Stx2a holotoxin is a ribosome-inactivating protein (RIP), which belongs to a family of AB5 toxins, consisting of a monomeric A subunit (Stx2A) and a pentameric B subunit (Stx2B). The catalytic A1 subunit of Stx2a (Stx2A1) interacts with the ribosomal P-stalk for loading onto the ribosome and depurination of the sarcin–ricin loop, which halts protein synthesis. The P-stalk is composed of five P-proteins, namely uL10 protein (former name P0) forming the base of the stalk, and two P1–P2 heterodimers, each binding to uL10 (9, 10). Stx2A1 (15, 16) as well as other RIPs bind to the conserved CTDs, with a prominent role of the CTDs from the P1 proteins.

Here, the state-of-the-art instrumentation and multiple software processing platforms were used to determine a 4.1 Å cryo-EM structure of the 72 kDa Stx2a in complex with the ribosomal P-stalk, with local resolutions in the range of 3.5 to 7.5 Å. Stx2A, denoted as chain A, is composed of two fragments, namely a catalytic Stx2A1 fragment consisting of the N-glycosidase active site and the P-stalk CTD-binding site, and Stx2A2 composed of an α-helix, which inserts into the channel formed by a pentameric ring of Stx2B. The structure reveals the presence of a density associated with Stx2a in the region identified earlier as the binding site for the CTD. This density can be fitted with the C-terminal six amino acids from a single P-protein of the P-stalk, denoted as chain P. The cryo-EM structure unveils that the six amino-acid peptide (GFGLFD) from the CTD interacts with Stx2a. The CTD-binding pocket is located on the opposite side of the Stx2a surface than the active site, and it is formed by α-helices: A, F, I, and loop 1 spanning residues Pro27–Ser39. The binding interface involves Stx2a residues previously implicated in the P11 binding by the X-ray structure and mutational analysis, such as Asn18, Thr35, Thr36, Ser229, Leu232, and the conserved Arg172, Arg176, and Arg179. Importantly, the cryo-EM structure reveals novel previously unidentified amino acids, involved in binding to the CTD, namely Gln10, Gln11, and Val14. The density representing the CTD in the cryo-EM structure can also be fitted with the six amino-acid peptide adopting an α-helical, rather than a random-coil conformation, as observed in the X-ray structure. The cryo-EM structure reveals a part of this loop spanning residues Cys241–His243 and Ser256–Cys260. The structure shows that Tyr77, located in the N-glycosidase active site, is occluded by Stx2A2.

> REFTIDFSTQQSYVSSLNSIRTEISTPLEHISQGTTSVSVINHTPPGSYFAVDIRGLDVYQARFDHLRLIIEQNNLYVAGFVNTATNTFYRFSDFTHISVPGVTTVSMTTDSSYTTLQRVAALERSGMQISRHSLVSSYLALMEFSGNTMTRDASRAVLRFVTVTAEALRFRQIQREFRQALSETAPVYTMTPGDVDLTLNWGRISNVLPEYRGEDGVRVGRISFNNISAILGTVAVILNCHHQGARSVRAVNEDSQPECQITGDRPVIKINNTLWESNTAAAFLNRKSQFLYTTGK;>[5x]ADCAKGKIEFSKYNEDDTFTVKVDGKEYWTSRWNLQPLLQSAQLTGMTVTIKSSTCESGSGFAEVQFNND;> GFGLFD>[2x]MAASGEPQRQWQEEVAAVVVVGSCMTDLVSLTSRLPKTGETIHGH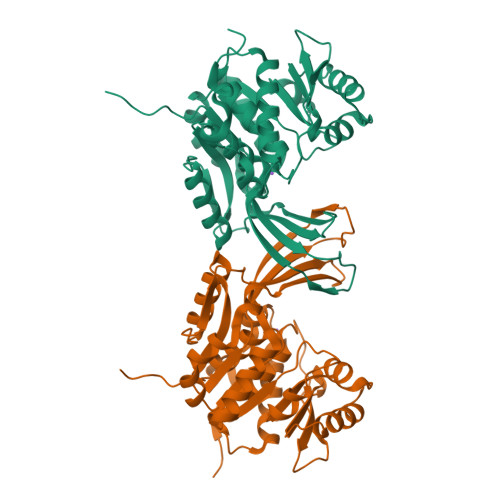KFFIGFGGKGANQCVQAARLGAMTSMVCKVGKDSFGNDYIENLKQNDISTEFTYQTKDAATGTASIIVNNEGQNIIVIVAGANLLLNTEDLRAAANVISRAKVMVCQLEITPATSLEALTMARRSGVKTLFNPAPAIADLDPQFYTLSDVFCCNESEAEILTGLTVGSAADAGEAALVLLKRGCQVVIITLGAEGCVVLSQTEPEPKHIPTEKVKAVDTTGAGDSFVGALAFYLAYYPNLSLEDMLNRSNFIAAVSVQAAGTQSSYPYKKDLPLTLFLEHHHHHH>VNQSETEIEILAEKIARWARARS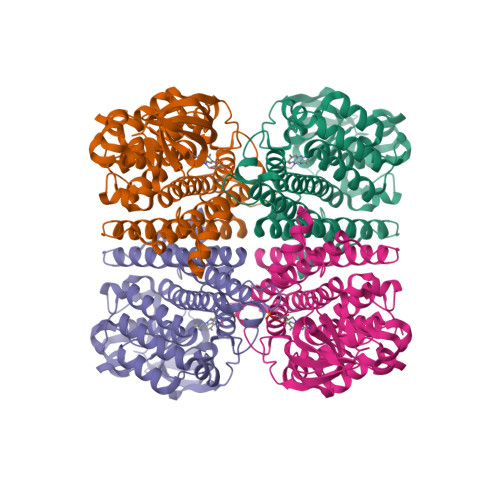AEIERDRRLPDELVTRLREAGLLRATMPREVAAPELAPGRALRCAEAVARGDASAGWCVSIAITSALLVAYLPARSREEMFGGGRGVAAGVWAPRGTARSVDGGVVVSGRWPFCSGINHADIMFAGCFVDDRQVPSVVALNKDELQVLDTWHTLGLRGTGSHDCVADDVFVPADRVFSVFDGPIVDRPLYRFPVFGFFALSIGAAALGNARAAIDDLVELAGGKKGLGSTRTLAERSATQAAAATAESALGAARALFYEVIEAAWQVSHDAEAVPVTMRNRLRLAATHAVRTSADVVRSMYDLAGGTAIYDNAPLQRRFRDAFTATAHFQVNEASRELPGRVLLDQPADVSML[4x]>MGDPERPEAAGLDQDERS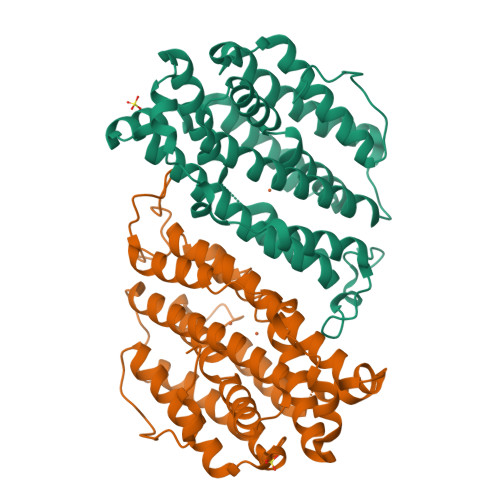SSDTNESEIKSNEEPLLRKSSRRFVIFPIQYPDIWKMYKQAQASFWTAEEVDLSKDLPHWNKLKADEKYFISHILAFFAASDGIVNENLVERFSQEVQVPEARCFYGFQILIENVHSEMYSLLIDTYIRDPKKREFLFNAIETMPYVKKKADWALRWIADRKSTFGERVVAFAAVEGVFFSGSFAAIFWLKKRGLMPGLTFSNELISRDEGLHCDFACLMFQYLVNKPSEERVREIIVDAVKIEQEFLTEALPVGLIGMNCILMKQYIEFVADRLLVELGFSKVFQAENPFDFMENISLEGKTNFFEKRVSEYQRFAVMAETTDNVFTLDADF[2x]>[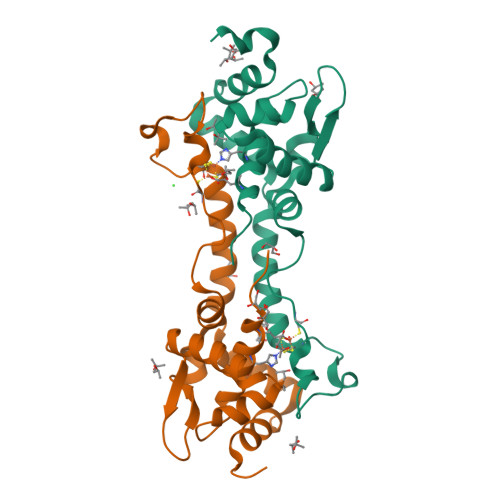8x]MKLSGGVEWALHCCVVLTAASRPVPAARLAELHDVSPSYLAKQMQALSRAGLVRSVQGKTGGYVLTRPAVEITLLDVVQAVDGPDPAFVCTEIRQRGPLATPPEKCTKACPIARAMGAAEAAWRASLAATTIADLVATVDDESGPDALPGVGAWLIEGLGHHHHHH>[5x]MYSTAVLLNKISPTRDGQTMTLADLQYLSFSELRKIFDDQLSWGEARHLYHETIEQKKNNRLLEARIFTRANPQLSGAIRLGIERDSVSRSYDEMFGARSSSFVKPGSVASMFSPAGYLTELYREAKDLHFSSSAYHLDNRRPDLADLTLSQSNMDTEISTLTLSNELLLEHITRKTGGDSDALMESLSTYRQAIDTPYHQPYETIRQVIMTHDSTLSALSRNPEVMGQAEGASLLAILANISPELYNILTEEITEKNADALFAQNFSENITPENFASQSWIAKYYGLELSEVQKYLGMLQNGYSDSTSAYVDNISTGLVVNNESKLEAYKITRVKTDDYDKNINYFDLMYEGNNQFFIRANFKVSREFGATLRKNAGPSGIVGSLSGPLIANTNFKSNYLSNISDSEYKNGVKIYAYRYTSSTSATNQGGGIFTFESYPLTIFALKLNKAIRLCLTSGLSPNELQTIVRSDNAQGIINDSVLTKVFYTLFYSHRYALSFDDAQVLNGSVINQYADDDSVSHFNRLFNTPPLKGKIFEADGNTVSIDPDEEQSTFARSALMRGLGVNSGELYQLGKLAGVLDAQNTITLSVFVISSLYRLTLLARVHQLTVNELCMLYGLSPFNGKTTASLSSGELPRLVIWLYQVTQWLTEAEITTEAIWLLCTPEFSGNISPEISNLLNNLRPSISEDMAQSHNRELQAEILAPFIAATLHLASPDMARYILLWTDNLRPGGLDIAGFMTLVLKESLNANETTQLVQFCHVMAQLSLSVQTLRLSEAELSVLVISGFAVLGAKNQPAGQHNIDTLFSLYRFHQWINGLGNPGSDTLDMLRQQTLTADRLASVMGLDISMVTQAMVSAGVNQLQCWQDINTVLQWIDVASALHTMPSVIRTLVNIRYVTALNKAESNLPSWDEWQTLAENMEAGLSTQQAQTLADYTAERLSSVLCNWFLANIQPEGVSLHSRDDLYSYFLIDNQVSSAIKTTRLAEAIAGIQLYINRALNRIEPNARADVSTRQFFTDWTVNNRYSTWGGVSRLVYYPENYIDPTQRIGQTRMMDELLENISQSKLSRDTVEDAFKTYLTRFETVADLKVVSAYHDNVNSNTGLTWFVGQTRENLPEYYWRNVDISRMQAGELAANAWKEWTKIDTAVNPYKDAIRPVIFRERLHLIWVEKEEVAKNGTDPVETYDRFTLKLAFLRHDGSWSAPWSYDITTQVEAVTDKKPDTERLALAASGFQGEDTLLVFVYKTGKSYSDFGGSNKNVAGMTIYGDGSFKKMENTALSRYSQLKNTFDIIHTQGNDLVRKASYRFAQDFEVPASLNMGSAIGDDSLTVMENGNIPQITSKYSSDNLAITLHNAAFTVRYDGSGNVIRNKQISAMKLTGVDGKSQYGNAFIIANTVKHYGGYSDLGGPITVYNKTKNYIASVQGHLMNADYTRRLILTPVENNYYARLFEFPFSPNTILNTVFTVGSNKTSDFKKCSYAVDGNNSQGFQIFSSYQSSGWLDIDTGINNTDIKITVMAGSKTHTFTASDHIASLPANSFDAMPYTFKPLEIDASSLAFTNNIAPLDIVFETKAKDGRVLGKIKQTLSVKRVNYNPEDILFLRETHSGAQYMQLGVYRIRLNTLLASQLVSRANTGIDTILTMETQRLPEPPLGEGFFANFVLPKYDPAEHGDERWFKIHIGNVGGNTGRQPYYSGMLSDTSETSMTLFVPYAEGYYMHEGVRLGVGYQKITYDNTWESAFFYFDETKQQFVLINDADHDSGMTQQGIVKNIKKYKGFLNVSIATGYSAPMDFNSASALYYWELFYYTPMMCFQRLLQEKQFDEATQWINYVYNPAGYIVNGEIAPWIWNCRPLEETTSWNANPLDAIDPDAVAQNDPMHYKIATFMRLLDQLILRGDMAYRELTRDALNEAKMWYVRTLELLGDEPEDYGSQQWAAPSLSGAASQTVQAAYQQDLTMLGRGGVSKNLRTANSLVGLFLPEYNPALTDYWQTLRLRLFNLRHNLSIDGQPLSLAIYAEPTDPKALLTSMVQASQGGSAVLPGTLSLYRFPVMLERTRNLVAQLTQFGTSLLSMAEHDDADELTTLLLQQGMELATQSIRIQQRTVDEVDADIAVLAESRRSAQNRLEKYQQLYDEDINHGEQRAMSLLDAAAGQSLAGQVLSIAEGVADLVPNVFGLACGGSRWGAALRASASVMSLSATASQYSADKISRSEAYRRRRQEWEIQRDNADGEVKQMDAQLESLKIRREAAQMQVEYQETQQAHTQAQLELLQRKFTNKALYSWMRGKLSAIYYQFFDLTQSFCLMAQEALRRELTDNGVTFIRGGAWNGTTAGLMAGETLLLNLAEMEKVWLERDERALEVTRTVSLAQFYQALSSDNFNLTEKLTQFLREGKGNVGASGNELKLSNRQIEASVRLSDLKIFSDYPESLGNTRQLKQVSVTLPALVGPYEDIRAVLNYGGSIVMPRGCSAIALSHGVNDSGQFMLDFNDSRYLPFEGISVNDSGSLTLSFPDATDRQKALLESLSDIILHIRYTIRS

Of these are a class of multi-protein ABC toxin complexes (Tcs) that have multiple receptor binding domains on the shell of the A subunit (TcA) for recognizing and binding target cells. The Xenorhabdus nematophilus TcA, XptA2, has thus far only displayed toxicity to insects. Here we report the high-resolution structure of the Xenorhabdus nematophilus TcA XptA2 by X-ray crystallography and cryo-EM, each at 3.1 Å resolution. XptA2 forms a 17.5-nm-wide, 24-nm-long pentamer with a molecular mass of ~1.4 megadaltons (MDa).

To generate a structure in the absence of crystal packing, we next solved the pre-pore structure of XptA2 using single particle cryo-EM, which yielded a map at 3.1 Å resolution. The cryo-EM and X-ray structures exhibit 5-fold internal symmetry comprising five protomers that assemble as a pentamer. XptA2 shares the conserved α-helical translocation channel that is less than 1 nm in diameter, housed within a balloon-shaped outer shell. The remaining β-sheets are composed of three IgG-like receptor binding domains (RBDs) that may play a role in cell surface receptor recognition and targeting. Both structures reveal that the RBDs are like sockets in grooves with only modest contact with the main XptA2 shell. The central translocation channel is formed by five extended α-helices per protomer for 25 α-helices. The XptA2 linker is disordered and “loose” in the pre-pore state between the translocation channel and the outer shell, like the TcdA1 linker. The unknown density most likely represents a counter-ion deriving from the crystallization conditions due to the absence of this ion in the cryo-EM structure.>HHGSTPVETHGQLSVKGGQLVDENGKPVQLRGMSSHGLQWFGDFVNKDSMKWLRDDWGINVFRVAMYTAEGGYITNPSVKNKVKEAVEAAIDLGMYVIIDWHILSDNDPNTYKEQAKAFFQEMAAKYG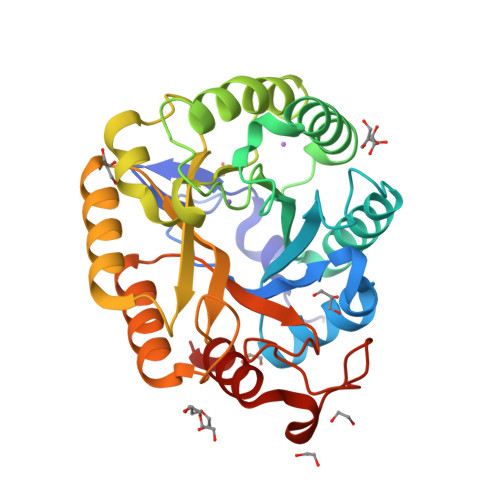NYPNVIYEICNEPNGGVTWSNQIKPYAEEVIPAIRANDPDNIIIVGTPTWSQDVHDAADNPLPYSNIMYALHFYAGTHGQSLRDKIDYALSKGVAIFVTEWGTSDASGNGGPFLNESQKWIDFMNSRNISWANWSLSDKSETSAALMPGASPTGGWTDSNLSASGKFVREQIRRS[6x]> SNAAPNISAYSDPYFNGANGLAQKDIIIRPANIELDAPAWVTMDYRTGDIVSE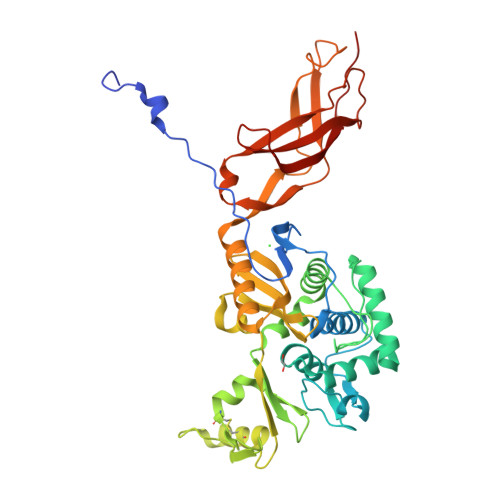KNMDVRRAPASLTKIMTSYIVASEIKAGNLSWDTMIPISENAASTGGSKMYVKAGAKVSVRNLVTGMDVVSGNDATIALAEYIGGTTQAFTDLMNQTAKAIGMNNTHFANPDGLPGGEQYTTAHDMALLARSYIYNFPEAYKVYDDKGLVWNATKQDSVSIADRKQCLPKFDRATGNVIESYTVKDLDDQAKDKCNKLFPKGDNFVLQNNRNRLLFTFDGADGMKTGHTDAAGYCLVSSAKQDGERFISVVLGTTSSAKRDSESAKLLRYALSKYENVLLYKANSPVTISADNIPNAKAGQKLTVASNQNIYKTVPKTYVPYLKQGIEFNPNLNAPIKTGQTVGNLVITLGDTKEEIASIPVVAMNNVSQKGWW>KRCLFVCRHGERMDVVFGKYWLSQCFDAKGRYIRTNLNMPHSLPQRSGGFRDYEKDAPI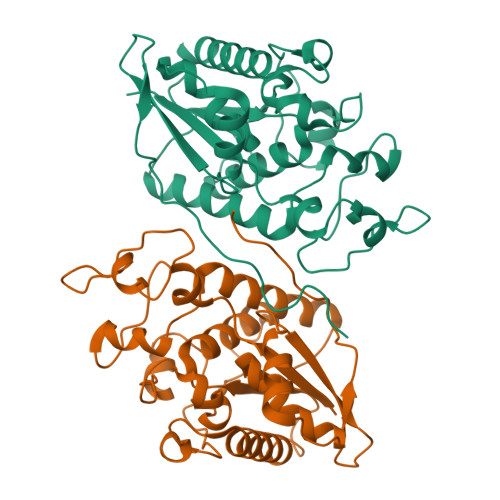TVFGCMQARLVGEALLESNTIIDHVYCSPSLRCVQTAHNILKGLQQENHLKIRVEPGLFEWTKWVAGSTLPAWIPPSELAAANLSVDTTYRPHIPISKLVVSESYDTYISRSFQVTKEIISECKSKGNNILIVAHASSLEACTCQLQGLSPQNSKDFVQMVRKIPYLGFCSCEELGETGIWQLTDPPILPLTHGPTGGFNWRE[3x]>[6x]ADFKFEPMRSLIYVDCVSEDYRPKLQRWIYKVHIPDSISQFEPYVTKYAFYPSFPIPPQGDRFGYARMQLTEHHWLVSDLDPRLEIKAIAETFPMDVLVWQGQIPAAAHTDAQIDSDGDAGNAARKSNNAEGNPFIFAFLPMWWEKDLKGKGRTIEDGANYRFNMTIGFPEGVDKAEGEKWLFEKVV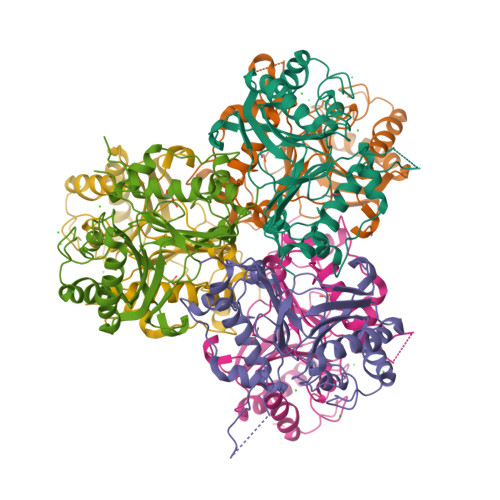PILQAAPECTRVLASAVKKDINGCVMDWVLEIWFENQSGWYKVMVDDMKALEKPSWAQQDAFPFLKPYHNVCSAAVADYTPSNNLANYRGYITMR> MQDAITAVINASDVQGKYLDTAAMEKLKAYFAT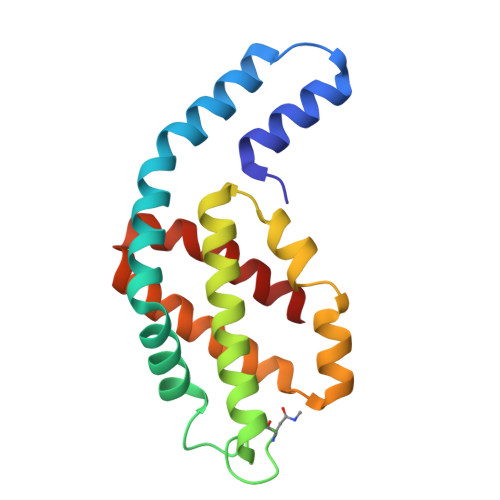GELRVRAASVISANAANIVKEAVAKSLLYSDITRPGGNMYTTRRYAACIRDLDYYLRYATYAMLAGDPSILDERVLNGLKETYNSLGVPIAATVQAIQAMKEVTASLVGADAGKEMGIYFDYICSGLS>GAMESKKRQWALEDFEIGRPLGKGKFGNVYLAREKQSKFILALKVLFKAQLEKAGVEHQLRR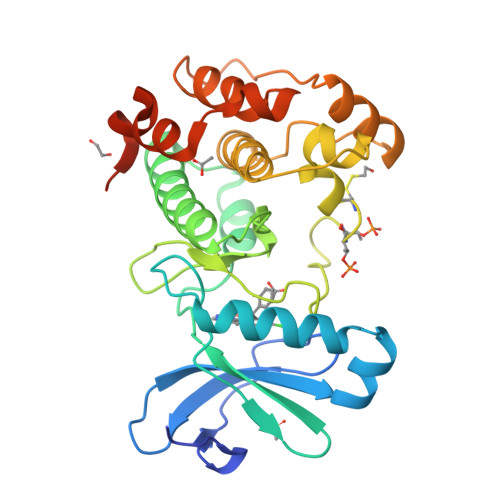EVEIQSHLRHPNILRLYGYFHDATRVYLILEYAPRGEVYKELQKLSKFDEQRTATYITELANALSYCHSKRVIHRDIKPENLLLGSAGELKIADFGWSVHAPSSRRTTLCGTLDYLPPEMIEGRMHDEKVDLWSLGVLCYEFLVGKPPFEANTYQETYKRISRVEFTFPDFVTEGARDLISRLLKHNPSQRPMLREVLEHPWITANSSKPSNCQNKESASKQS[4x]3-[3-(4-decylphenyl)-1,2,4-oxadiazol-5-yl]propan-1-amine | C21 H33 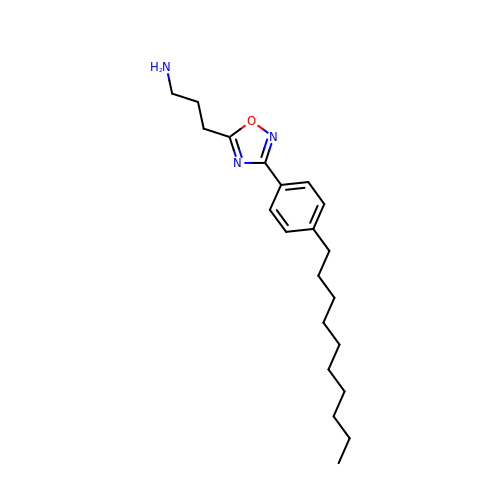N3 O | VLTITRMWGPJCFJ-UHFFFAOYSA-N>HHHHHHFNLPAGNYKLPKLLYCSNGGHFLRILPDGTVDGTRDRSDQHIQ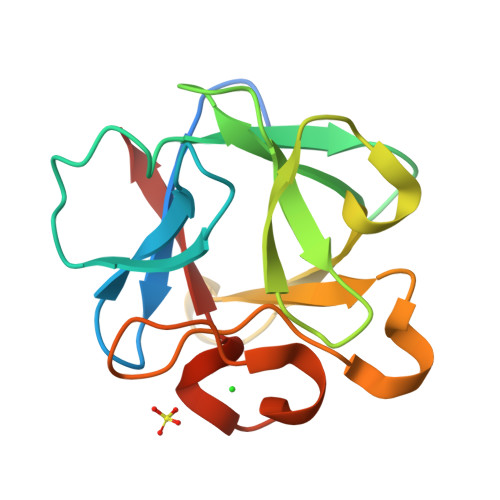LQLSAESVGEVYIKSTETGQYLAMDTDGLLYGSQTPSEECLFLERLEENHYNTYTSKKHAEKNWFVGLKKNGSCKRGPRTHYGQKAILFLPLPVSSD[2x]>NGPSPNLPPGFDFTDPAIYAERLPVAEFAELRSAAPIWWNGQDPGKGGGFHDGGFWAITKLNDVKEISRHSDVFSSYENGVIPRFKNDIAREDIEVQRFVMLNMDAPHHTRLRKIISRGFTPRAVGRLHDELQERAQKIAAEAAAAGSGDFVEQVSCELPLQAIAGLLGVPQEDRGKLFHWSNEMTGNEDPEYAHIDPKASSAELIGYAMKMAEEKAKNPADDIVTQLIQADIDGEKLSDDEFGFFVVMLAVAGNETTRNSITQGMMAFAEHPDQWELYKKVRPETAADEIVRWATPVTAFQRTALRDYELSGVQIKKGQRVVMFYR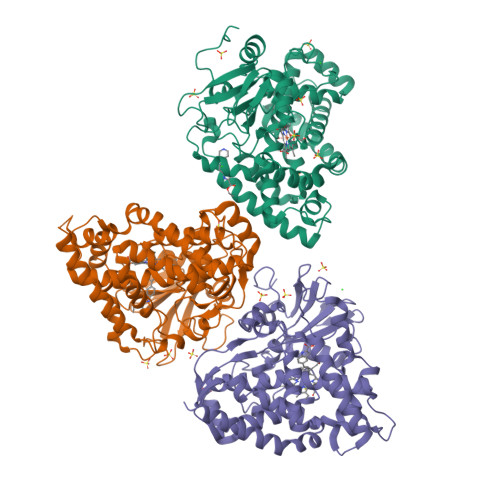SANFDEEVFQDPFTFNILRNPNPHVGFGGTGAHYCIGANLARMTINLIFNAVADHMPDLKPISAPERLRSGWLNGIKHWQVDYTGRCPVA[3x]>[2x]GA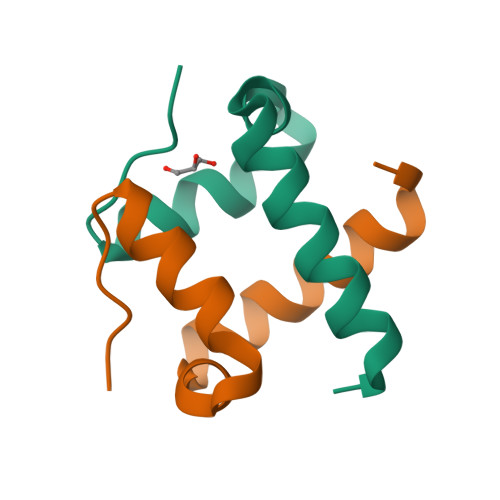MDPRKVSELRAFVKMCRQDPSVLHTEEMRFLREWVESMGGKVPP>SFELPALPYAKDALAPHISAETIEYHYGKHHQTYVTNLNNLIKGTAFEGKSLEEIIRSSEGGVFNNAAQVWNHTFYWNCLAPNAGGEPTGKVAEAIAASFGSFADFKAQFTDAAIKNFGSGWTWLVKNSDGKLAIVSTSNAGTPLTTDATPLLTVDVWEHAYYIDYRNARPGYLEHFWALVNWEFVAKNLA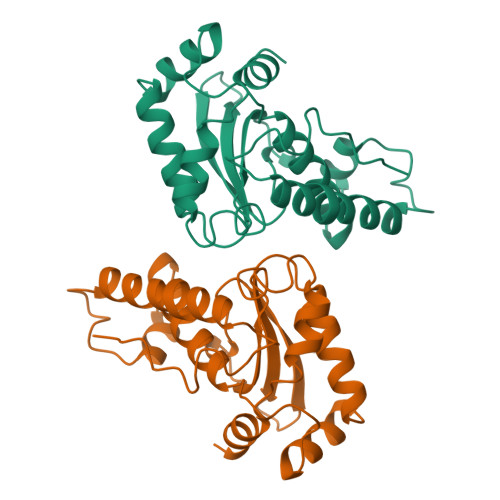A[2x]>GMEGEEYDKILVLNFGSQYFHLIVKRLNNIKIFSETKDYGVELKDIKDMNIKGVILSGGPYSVTEAGSPHLKKEVFEYFLEKKIPIFGICYGMQEIAVQMNGEVKKSKTSEYGCTDVNILRNDNINNITYCRNFGDSSSAMDLYSNYKLMNETCCLFENIKSDITTVWMNHNDEVTKIPENFYLVSSSENCLICSIYNKEYNIYGVQYHPEVYESLDGELMFYNFAYNICKCKKQFDPIRYHELELKNIEKYKHDHYVIAAMSGGIDSTVAAAYTHKIFKERFFGIFIDNGLLRKNEAENVYTFLKSTFPDMNITKIDASENFLSNLQGVTDPEQKRKIIGKLFIEEFEKAVNNIDIDINKTFLLQGTLYPDIIESKCSKNLSDTIKTHHNVGGLPKNLKFKLFEPFKYLFKDDVKTLSRELNLPEEITNRHPFPGPGLAIRVIGEINKHKLNILREVDDIFINDLKQYGLYNQISQAFAVLLSSKSVGVRGDARSYDYVCVLRAVKTSSFMTANWYQIPYDILDKITTRILSEVKGVNRILYD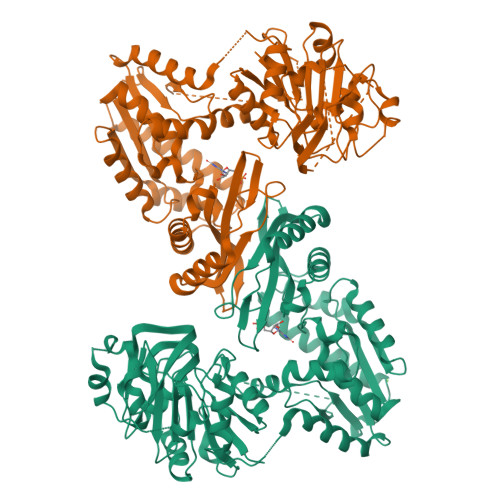VSSKPPATIEFE[2x]>[2x]AQTVPYGIPLIKADKVQAQGFKGANVKVAVLDTGIQASHPDLNVVGGASFVAGEAYNTDGNGHGTHVAGTVAALDNTTGVLGVAPSVSLYAVKVLNSSGSGSYSGIVSGIEWATTNGMDVINMSLGGASGSTAMKQAVDNAYARGVVVVAAAGNSGSSGNTNTIGYPAKYDSVIAVGAVDSNSNRASFSSVGAELEVMAPGAGVYSTYPT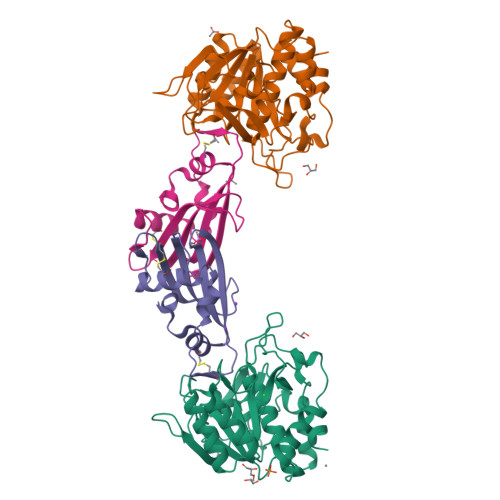NTYATLNGTSMASPHVAGAAALILSKHPNLSASQVRNRLSSTATYLGSSFYYGKGLINVEAAAQ;>GSAHGPSAMVFTVIQGSGEPTDTVLRATTLSCAYTAEGTHPAPRAACDALNATDGELNRLLAAPDPSLVCPMYFDPVTVTADGVLNGRRVAWKHTFSNTCVMSANLNSNPVYAF[2x]> MAEIPKEMLRAQTNVILLNVLKQGDNYVYGIIKQVKEASNGEMELNEATLYTIFKRLEKDGIISSYWGDESQGGRRKYYRLTEIGHENMRLAFESWSRV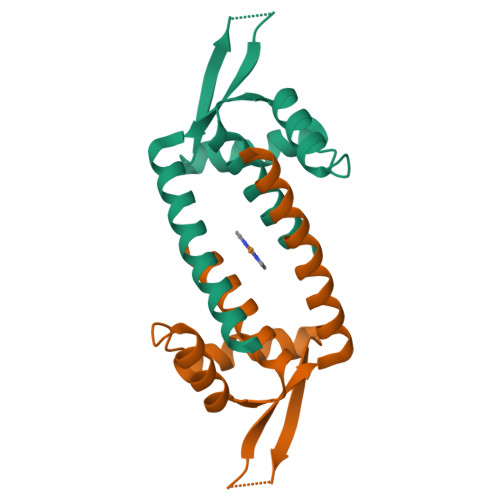DKIIENLEANKKSEAIKSRWSHPQFEK> MAEKTFKVVSDSGIHAR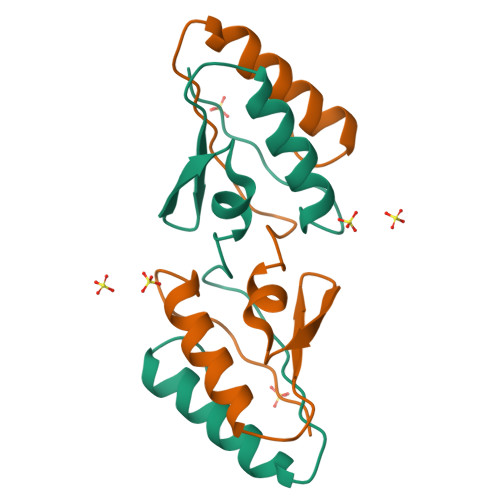PATILVQTASKWNSEIQLEYNGKTVNLKSIMGVMSLGIPKGATIKITAEGADAAEAMAALTDTLAKEGLAE> GSHMASMKKKGSVVIVGRINLSGDTAYAQQTRGEEGCQETSQTGRDKNQVEGE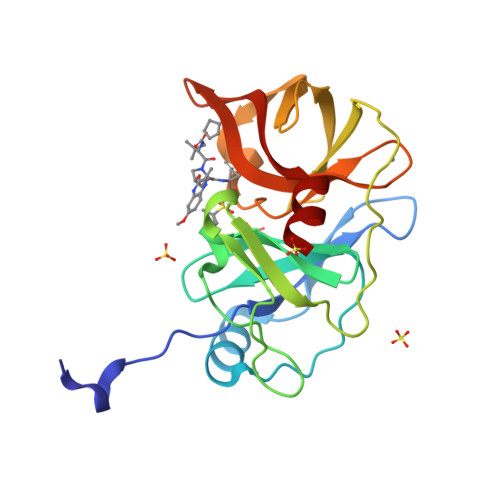VQIVSTATQTFLATSINGVLWTVYHGAGTRTIASPKGPVTQMYTNVDKDLVGWQAPQGSRSLTPCTCGSSDLYLVTRHADVIPVRRRGDSRGSLLSPRPISYLKGSSGGPLLCPAGHAVGIFRAAVCTRGVAKAVDFIPVESLETTMR> MAWPKVQPEVNIGVVGHVDHGKTTLVQAITGIWTSKHSEELKRGMTIKLGYAETNIGVCESCKKPEAYVTEPSCKSCGSDDEPKFLRRISFIDAPGHEVLMATMLSGAALMDGAILVVAANEPFPQPQTREHFVALGIIGVKNLIIVQNKVAVVSKEEALSQYRQIKQFTKGTWAENVPIIPVSALHKINIDSLIEGIEEYIKTPYRDLSQKPVMLVIRSFDVNKPGTQFNELKGGVIGGSIIQGLFKVDQEIKVLPGLRVEKQGKVSYEPIFTKISSIRFGDEEFKEAKPGGLVAIGTYLDPSLTKADNLLGS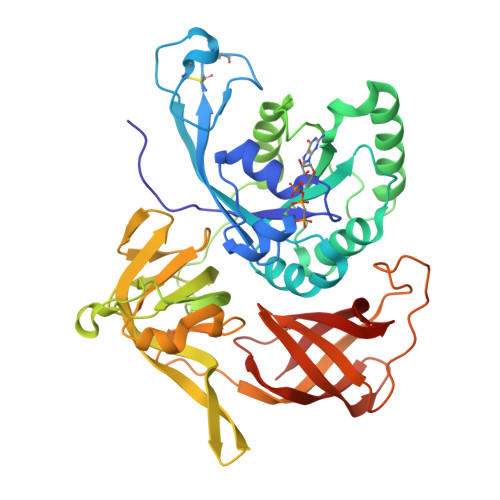IITLADAEVPVLWNIRIKYNLLERVVGAKEMLKVDPIRAKETLMLSVGSSTTLGIVTSVKKDEIEVELRRPVAVWSNNIRTVISRQIAGRWRMIGWGLVEI>UAUGUAACUCCGCCUAUGUCAUCUUA[4x];>[4x]GUAAAUGAUAUAGCCGGUCCCAAGCCCGGAAA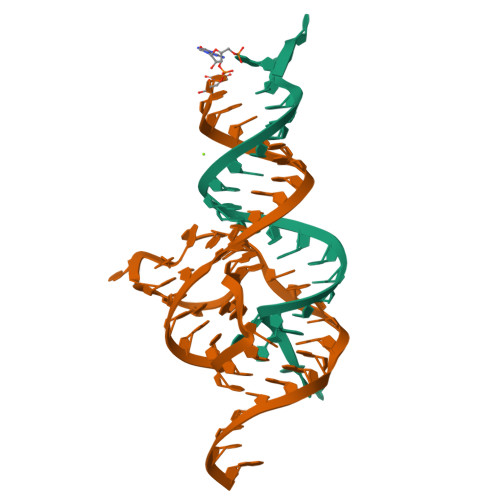AAGGAGGAGGGUAUA>[2x]GAMNWTVDIPIDQLPSLPPLPTDLRTRLDAALAKPAAQQPTWPADQALAMRTVLESVPPVTVPSEIVRLQEQLAQVAKGEAFLLQGGDCAETFMDNTEPHIRGNVRALLQMAVVLTYGASMPVVKVARIAGQYAKPRSADIDALGLRSYRGDMINGFAPDAAAREHDPSRLVRAYANASAAMNLVRALTSSGLASLHLVHDWNREFVRTSPAGARYEALATEIDRGLRFMSACGVADRNLQTAEIYASHEALVLDYERAMLRLSDGDDGEPQLFDLSAHTVWIGERTRQIDGAHIAFAQVIANPVGVKLGPNMTPELAVEYVERLDPHNKPGRLTLVSRMGNHKVRDLLPPIVEKVQATGHQVIWQCDPMHGNTHESSTGFKTRHFDRIVDEVQGFFEVHRALGTHPGGIHVEITGENVTECLGGAQDISETDLAGRYETACDPRLNTQQSLELAFLVAEMLRD

The enzyme 3-deoxy-d-arabino-heptulosonate 7-phosphate synthase (DAH7PS) catalyzes the first committed step of the shikimate pathway, which is the aldol-like condensation of phosphoenolpyruvate (PEP) and erythrose 4-phosphate (E4P) to produce 3-deoxy-d-arabino-heptulosonate 7-phosphate (DAH7P). Previous studies revealed a sophisticated synergistic allosteric regulation of DAH7PS from Mycobacterium tuberculosis (MtuDAH7PS) by binary or ternary combinations of the three aromatic amino acids, Phe, Tyr and Trp. The crystal structure of MtuDAH7PS revealed that the quaternary structure of this enzyme is a homotetramer of (β/α)8 TIM barrel subunits. Crystal structures of MtuDAH7PS in complex with different combinations of aromatic amino acids revealed three distinctive allosteric binding sites located at the dimer and tetramer interfaces of the enzyme, formed by accessory elements to the basic barrel.

The binding modes of all three aromatic d-amino acids in the Phe site are very similar to the binding modes of the respective l-enantiomers. The configuration of the ligand does not appear to significantly influence the conformation of the MtuDAH7PS residues that form the Phe binding site. For all aromatic d-amino acids, the amino and carboxy moieties project into the same binding pockets as the respective moieties of the l-amino acids. d-Phe binds to the Phe site in a very similar binding mode as the l-enantiomer, the root mean square deviation (RMSD) between the position of d-Phe and l-Phe ligands is 1.46 Å. The phenyl side chain of d-Phe is slightly tilted in the hydrophobic pocket when compared to the binding mode of l-Phe. However, high atomic displacement factors and poor electron density for the N-terminal region in the d-Trp bound structure suggest that flexibility of this region might be increased upon ligand binding. The only major difference in binding mode when comparing aromatic amino acids of l-configuration with their respective d-enantiomers is the lack of a hydrogen bonding interaction between the amino moiety of the d-configured ligands and the sidechain carbonyl of Asn175 on MtuDAH7PS (highlighted in red in Fig 4). The distance of the amino group of the ligand to the side-chain carbonyl group of Asn175 increases from 2.8 Å to 3.6 Å (l-Phe versus d-Phe), 2.6 Å to 3.7 Å (l-Trp versus d-Trp) and 2.7 Å to 3.6 Å (l-Tyr versus d-Tyr), respectively. The only significant difference between the binding mode of l-Phe and d-Phe in site 1 is the lack of a hydrogen bond between d-Phe and the Asn175 side-chain carbonyl. This may indicate that the ligand in site 1 needs to establish a contact to Asn175 in order for transmission of a signal from site 1 to either site 2 or the active site to occur. The affinity of d-Phe to the enzyme is only slightly lower when compared with the natural enantiomer: the dissociation constant (Kd) of d-Phe from MtuDAH7PS was determined as 93 ± 5 μM.> GHMGGDSEIQYLLEKLKKLEEDYYKLRELYRRLEDEKKFIESERIRYEREVRRLRSEVERLRSPPLLVGVVSDILEDGRVVVKSSTGPKFVVNTSQYINEEELKPGARVALNQQTLAIVNVLPTSKDPMVYGFEVEEKPEVSYEDIGGLDVQIEEIREAVELPLLKPELFAEVGIEPPKGVLLYGPPGTGKTLLAKAVANQTRATFIRVVGSEFVQKYIGEGARLVREVFQLAKEKAPSIIFIDELDAIA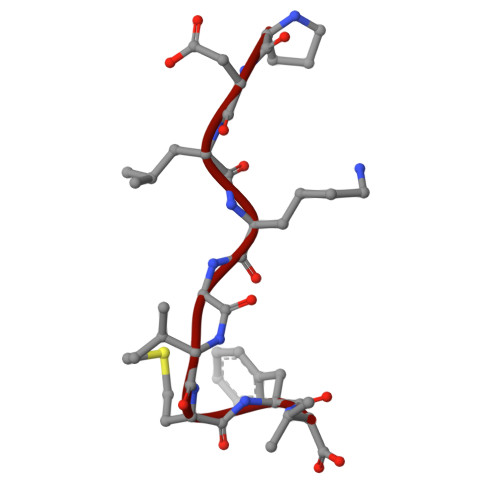ARRTNSDTSGDREVQRTMMQLLAELDGFDPRGDVKVIGATNRIDILDPAILRPGRFDRIIEVPLPTFEGRIQIFKIHTRKMKLAEDVDFKELARITEGASGADIKAICTEAGMFAIREERAKVTMLDFTKAIEKVLKKTTPIPDLKGVMFV1-tert-butyl-3-(naphthalen-1-yl)-1H-pyrazolo[3,4-d]pyrimidin-4-amine | C19 H19 N5 | 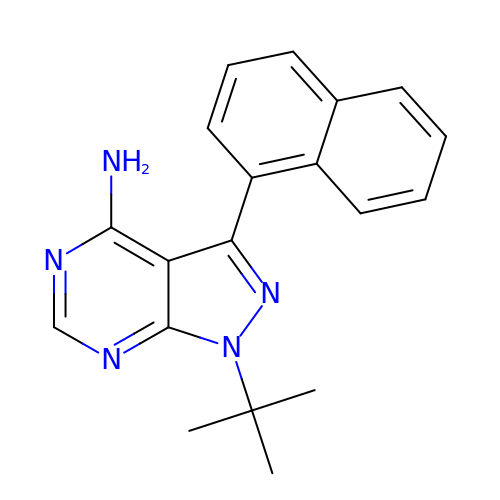XSHQBIXMLULFEV-UHFFFAOYSA-N>[6x]MRGSHHHHHHGSMDKNIIIGAMTALITPFKNGKVDEQSYARLIKRQIENGIDAVVPVGTTGESATLTHEEHRTCIEIAVETCKGTKVKVLAGAGSNATHDAVGLAKFAKEHGADGILSVAPYYNKPTQQGLYEHY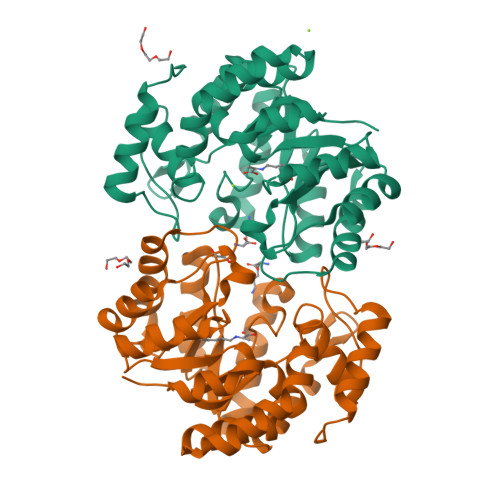KAIAQSVDIPVLLYNVPGRTGCEISTDTIIKLFRDCENIYGVKEASGNIDKCVDLLAHEPRMMLISGEDAINYPILSNGGKGVISVTSNLLPDMISALTHFALDENYKEAKKINDELYNINKILFCESNPIPIKTAMYLAGLIESLEFRLPLCSPSKENFAKIEEVMKKYKIKGF>[4x]MNLKDKILGVAKELFIKNGYNATTTGEIVKLSESSKGNLYYHFKTKENLFLEILNIQESKWQEQWKKEQIKAKTNREKFYLYNELSLTTEYYYPLQNAIIEFYTEYYKT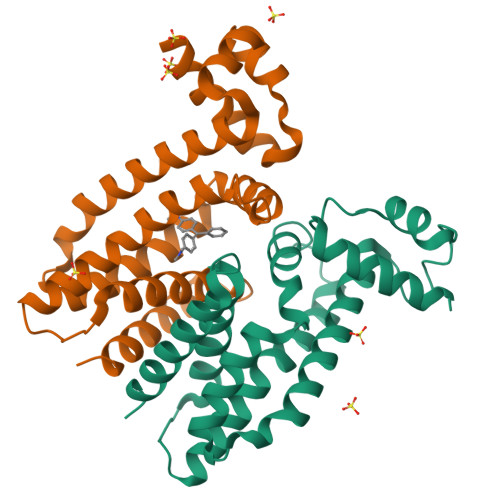NSINEKMNKLENKYIDAYHVIFKEGNLNGEWSINDVNAVSKIAANAVNGIVTFTHEQNINERIKLMNKFSQIFLNGLSK>[4x]MNELYQLEKEPIVGAET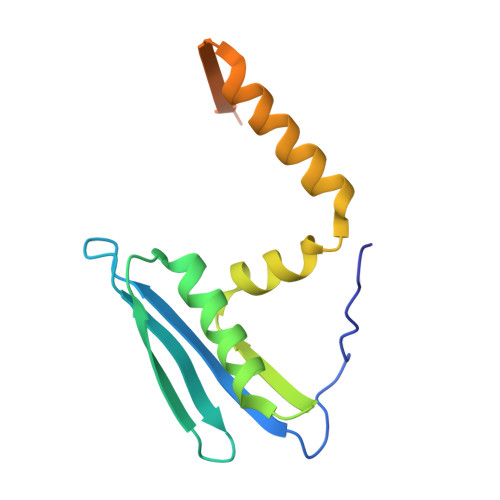FYVDGAANRETKLGKAGYVTNRGRQKVVTLTDTTNQKTELQAIYLALQDSGLEVNIVTDSQYALGIIQAQPDQSESELVNQIIEQLIKKEKVYLAWVPAHKGIGGNEQVDKLVSAGIRKVL>[3x]GMERAAFGKLVQALRREHRDEKGRVWTQEVLAERTQLPKRTIERIENGSLAHLDADILLRLADALELTIGERREFFFAATGIIEQKSATYKRSPEESLQYLIDMIRNMNVPAFVTDQYVNIIAANMITIRFFNIPMELIETAPLLPHGYNLMRVVFGTEYDFRRVVGTMWDEVARHNMQLFRAISLRVRADGYFVELLDNLMQYREFKRFWERAHLETEDTSAENFWYQYTHPVYGLLSYVSSRSQIPTSMGLLSMHTYIPLSPATTDLFAKLSTVANQDVIRLAPWPRSNG

MltR functions as a dimer, where each monomer consists of an N-terminal DNA-binding domain with an HTH (helix-turn-helix) motif and a C-terminal PAS-like (Per-Arnt-Sim) domain, which is involved in ligand binding. MltR consists of two domains, a small helical DNA-binding domain (DBD, residues 1-80) and a larger α/β C-terminal ligand-binding domain (LBD, residues 92–291). The C-terminal domain adopts a fold that is related to the PAS domain and binds a putative myristic acid at the expected ligand-binding site. In conclusion, we have determined the crystal structure of a novel transcription factor that is a representative of a large group of regulators with significant implications in antibiotic production and fatty-acid biosynthesis.

The crystal structure of MltR was determined in space group C2 using the SAD method, and was refined to a resolution of 2.3 Å with an Rcryst of 0.168 and an Rfree of 0.206. The asymmetric unit (asu) contains three monomers (1.5 dimers), which are similar to each other (average rmsd 0.7 Å for 289 Cα atoms). Each monomer contains residues 0 to 291 (residue Gly0 is the residue that remains after cleavage of the N-terminal purification tag) and one fatty acid tentatively assigned as myristic acid (MYR). In the first dimer, the two monomers (chains A and B) are related by a non-crystallographic two-fold axis, whereas the second dimer is formed by monomers (chains C and C’) that are related by the crystallographic two-fold axis. Each dimer is arranged in a side-to-side arrangement with the DBDs at one end and the LBDs at the other, resulting in a relatively flat arrangement with molecular dimension of 75 Å × 73 Å × 48 Å. The distance between the recognition helices (H3) in the MltR dimer is approximately 34 Å, enabling the two recognition helices to fit into successive DNA major grooves by spanning ∼10 bp (1 turn of B-form DNA), and recognizing a two-fold symmetric DNA target (palindrome or pseudo-palindrome). Although MltR was crystallized without the addition of any substrate, additional electron density in the putative ligand-binding site clearly indicated the presence of a fatty acid-type ligand, which was modeled as myristic acid (MYR) based on clear, interpretable electron density. MYR interacts favorably with the protein such that its carboxyl group is stabilized by hydrogen bonding interactions with Tyr227, Tyr258, and Asn176, and its hydrophobic tail is surrounded by hydrophobic side chains in the interior of the protein. The cavity is not accessible from the protein surface by molecules larger than water. Thus, conformational changes are required for MYR (or other ligands) to gain access to the binding site.> GPVEDAITAAIGRVADTVGTGPTNSEAIPALTAAETGHTSQVVPSDTMQTRHVKNYHSRSESTIENFLCRSACVYFTEYENSGAKRYAEWVITPRQAAQLRRKLEFFTYVRFDLELTFVITSTQQPSTTQNQDAQILTHQIMYVPPGGPVPDKVDSYVWQTSTNPSVFWTEGNAPPRMSVPFLSIGNAYSNFYDGWSEFSRNGVYGINTLNNMGTLYARHVNAGSTGPIKSTIRIYFKPKHVKAWIPRPPRLCQYEKAKNVNFQPSGVTTTRQSITTMTNT;> SPTVEECGYSDRVRSITLGNSTITTQECANVVVGYGVWPDYLKDSEATAEDQPTQPDVATCRFYTLDSVQWQKTSPGWWWKLPDALSNLGLFGQNMQYHYLGRTGYTIHVQCNASKFHQGCLLVVCVPEAEMGCATLNNTPSSAELLGGDTAKEFADKPVASGSNKLVQRVVYNAGMGVGVGNLTIFPHQWINLRTNNSATIVMPYTNSVPMDNMFRHNNVTLMVIPFVPLDYCPGSTTYVPITVTIAPMCAEYNGLRLAGHQ;> GLPTMNTPGSCQFLTSDDFQSPSAMPQYDVTPEMRIPGEVKNLMEIAEVDSVVPVQNVGEKVNSMEAYQIPVRSNEGSGTQVFGFPLQPGYSSVFSRTLLGEILNYYTHWSGSIKLTFMFCGSAMATGKFLLAYSPPGAGAPTKRVDAMLGTHVVWDVGLQSSCVLCIPWISQTHYRYVASDEYTAGGFITCWYQTNIVVPADAQSSCYIMCFVSACNDFSVRLLKDTPFISQENFFQ;> GAQVSTQKTGAHETGLNASGNSIIHYTNINYYKDAASNSANRQDFTQDPSKFTEPVKDIMIKSLPALN;> SITTPEEMIEKAKGETAYLPCKFTLSPEDQGPLDIEWLISPADNQKVDQVIILYSGDKIYDDYYPDLKGRVHFTSNDLKSGDASINVTNLQLSDIGTYQ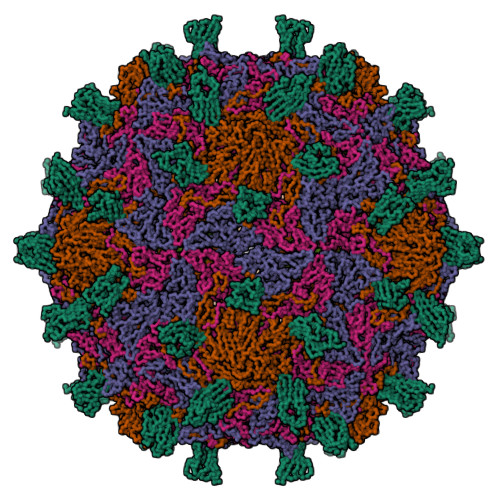CKVKKAPGVANKKIHLVVLVK> MTFEEKLSKIYNEIANEISSMIPVEWEKVYTMAYIDDGGGEVFFNYTKPGSDDLNYYTNIPKEYNISVQVFDDLWMDLYDLFEELRDLFKEEDLEPWTSCEFDFTREGELKVSFDYIDWINSEFGQIGRQNYYKYRKFGILPETEYEINKVKEIEQYIKELE;> PNYTKVEFGEHYARLRPKKLKANIEYTTPTGHIYRTDHKGRIKEVYVDNLSLKDGDRNSHAQRTVGGEDRLPDDDGGHLIARMFGGSKDIDNLVAQS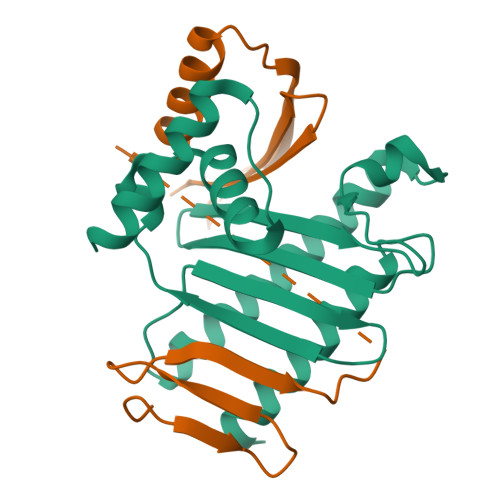KFINRPFKEKGHWYNLEKEWQEFLNSGKEVKNIKMEVKYSGNSQRPTIFKVEYEINGERNIRRILNK> GPGSELPQMVQQLNSPDQQELQSALRKLSQIASGGNEQIQAV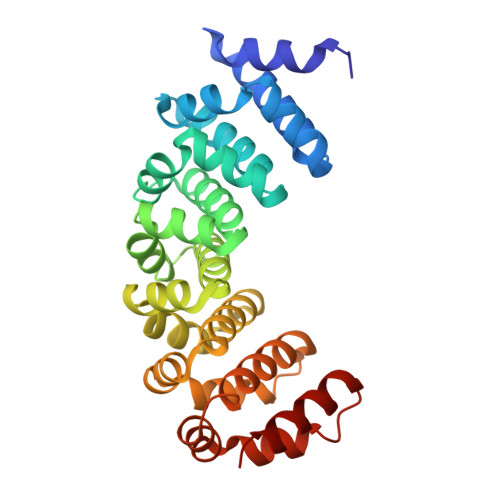IDAGALPALVQLLSSPNEQILQEALWTLGNIASGGNEQIQAVIDAGALPALVQLLSSPNEQILQEALWTLGNIASGGNEQIQAVIDAGALPALVQLLSSPNEQILQEALWTLGNIASGGNEQIQAVIDAGALPALVQLLSSPNEQILQEALWTLGNIASGGNEQIQAVIDAGALPALVQLLSSPNEQILQEALWTLGNIASGGNEQKQAVKEAGAEPALEQLQSSPNEKIQKEAQEALEKIQ> MGAKLAKTLQRFENKIKAGDYYEAHQTLRTIANRYVRSKSYEHAIELISQGAL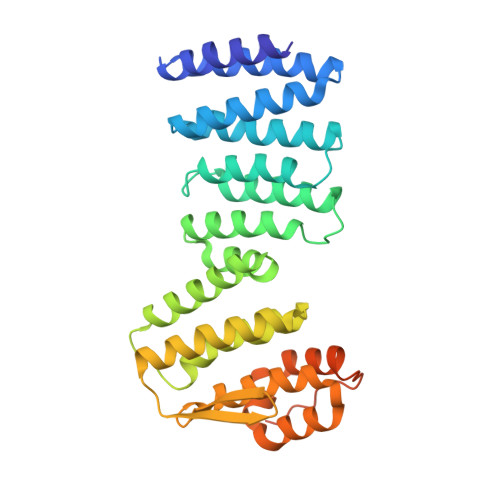SFLKAKQGGSGTDLIFYLLEVYDLAEVKVDDISVARLVRLIAELDPSEPNLKDVITGMNNWSIKFSEYKFGDPYLHNTIGSKLLEGDFVYEAERYFMLGTHDSMIKYVDLLWDWLCQVDDIEDSTVAEFFSRLVFNYLFISNISFAHESKDIFLERFIEKFHPKYEKIDKNGYEIVFFEDYSDLNFLQLLLITCQTADASYFLNLKNHYLDFSQAYKSELEFLGQEYFNIVAPKQTNFLQDMMSGFLGGSGENLYFQSLEHHHHHH>GSHMPTAIESCMVKFELSSSKWHMTSPKPHC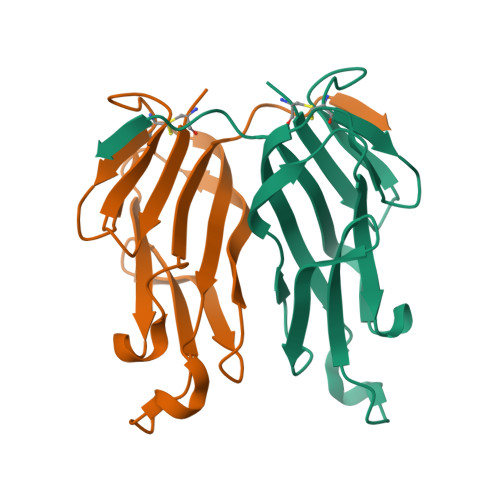VNTTSDGKLKILQSGTYLIYGQVIPVDKKYIKDNAPFVVQIYKKNDVLQTLMNDFQILPIGGVYELHAGDNIYLKFNSKDHIQKTNTYWGIILMPDLPFIS[2x]maslinic 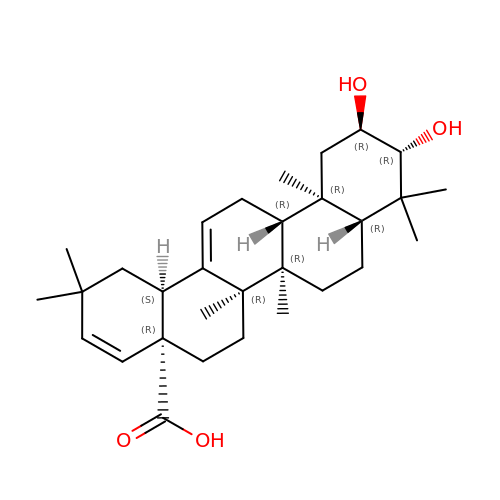acid | C30 H46 O4 | WZHVXLHLQLNEQU-LLICELPBSA-N>AAPTATVTPS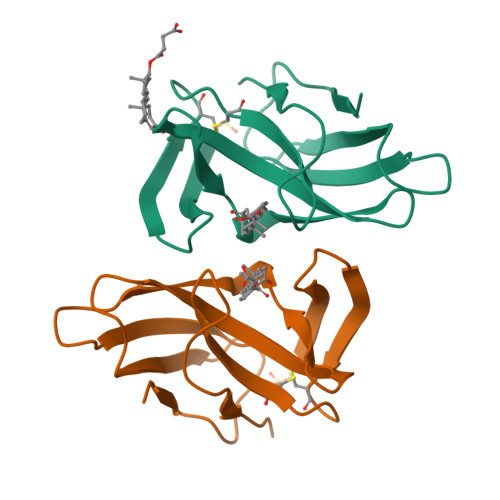SGLSDGTVVKVAGAGLQAGTAYWVYQRAAVDTGVHASNPADLSSVTADANGSASTSLTVRRSFEGFLFDGTRWGTVDCTTAACQVGLSDAAGNGPEGVAISFNH[6x]>GSVDVPVTDAYWQILFSVLKVTRNLKELDLSGNSLSHSAVKSLCKTLRRPRCLLETLRLAGCGLTAEDCKDLAFGLRANQTLTELDLSFNVLTDAGAKHLCQRLRQPSCKLQRLQLVSCGLTSDCCQDLASVLSASPSLKELDLQQNNLDDVGVRLLCEGLRHPACKLIRLGLDQTTLSDEMRQELR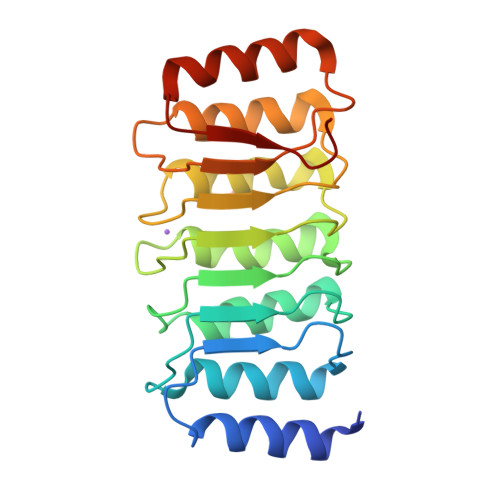ALEQEKPQLLIFSRRKPS[4x]>[3x]MENSADNLKYVCKDIKKIDDCLQIDTIYTGVCSDDTLYSDYCPMKNGKKGQCETNNDKISAGFIWLLVMFEHICDDDECSQNEKDQ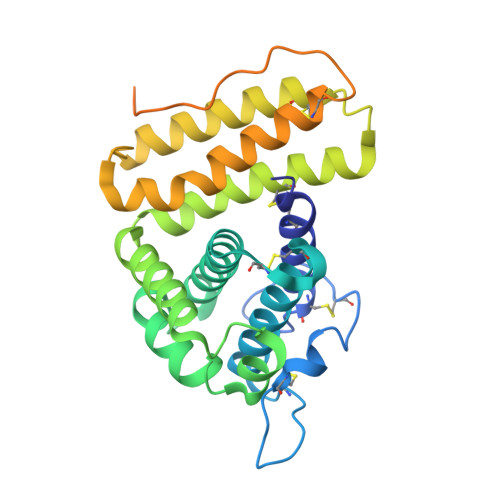YAGYAILWLSYILNQMPNEGIHTLKNFYTNHIETNTNYASHVSSASDSNYKGIVDKKIDLMNMNKAIIPKFYDIFKSLCNMYNELDKNEANYANCLKDAQNFVDEYQKFLNDNNVDTDDSSYKQILPILSNGYDNLIKKCNNGQHSNFPPLPTTKTTQLSAHISEDTSSSSSIASKLIPTLLIFAIPVFLGIAYKYSLFGFDKRFRRKYSREKLKNKE2-[(4-chloranyl-6-methoxy-pyrimidin-2-yl)carbamoylsulfamoyl]benzoic acid | 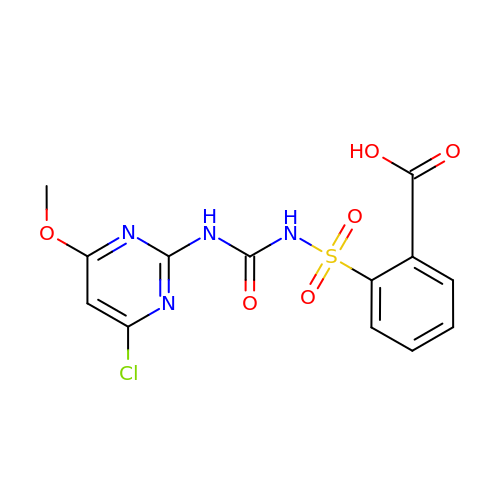C13 H11 Cl N4 O6 S | RIUXZHMCCFLRBI-UHFFFAOYSA-N> MTTPPLLQLPVEVKKTELNGFWDTGAQITCIPEAFLKEEIPIGEAQIKTLHGTKLQSVYYLKFKVLGRKVEAEVTTSPFDYVIISPSDIPWYKPQPLELTVKLPVQDFKKELINKANINNEEKKQLAKLLDKYDVLWQQWENQVGHRKIPPHNIATGTVAPRPQRQYHINTKAKPSIQQVIDDLLKQGVLIKQTSVMNTPIYPVPKPDGKWRMVLDYRAVNKTVPLIGAQNQHSLGILTNLVRQKYKSTIDLSNGFWAHPITKDSQWITAFTWEGKQHVWTRLPQGFLNSPALFTADVVDLLKNIPGISVYVDDIYFSTETVSEHLKILEKVFKILLEAGYIVSLKKSALLRYEVTFLGFSITQTGRGLTSEFKDKIQNITSPRTLKELQSILGLFNFARNFVPNFSEIIKPLYSLISTAEGNNIKWTSEHTRYLEEIVSALNHAGNLEQRDNESPLVVKLNASPKTGYIRYYNKGGQKPIAYASHVFTNTELKFTPLEKLLVTMHKALIKAIDLALGQPIEVYSPIISMQK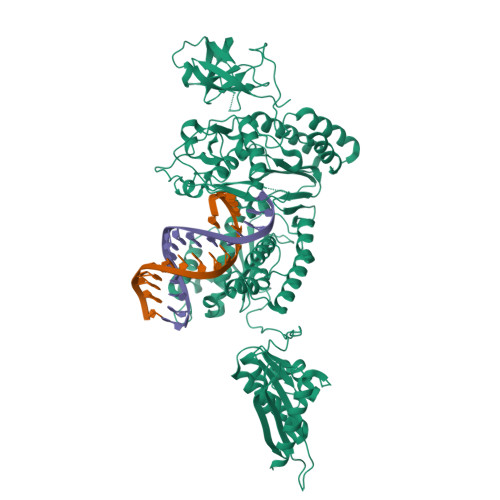LQKTPLPERKALSTRWITWLSYLEDPRITFYYDKTLPDLKNVPETVTDKKPKMLPIIEYAAVFYTNGSAIRSPDKNKSHSSGMGIVHAVFKPELTIEHQWSIPLGDHTAQYAEISAVEFACKKANNISGPVLIVTNSDYVARSVNEELPFWRSNGFVNNKKKPLKHISKWKNISDSLLLKRDIIIVHEPGHKPSYTSIHTQGNNLADKLATQGSYTVNNI>[2x]SMEMRAVVLAGFGGLNKLRLFRKAMPEPQDGELKIRVKACGLNFIDLMVRQGNIDNPPKTPLVPGFECSGIVEALG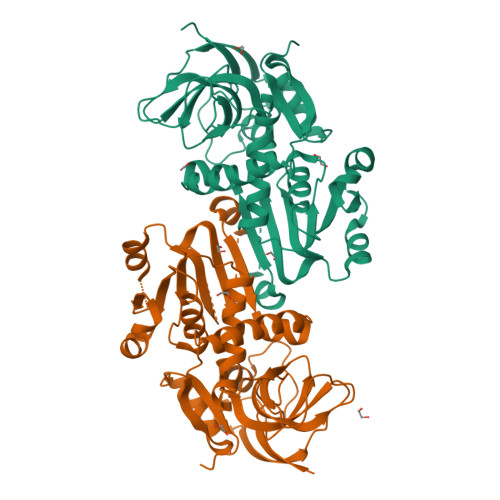DSVKGYEIGDRVMAFVNYNAWAEVVCTPVEFVYKIPDDMSFSEAAAFPMNFVTAYVMLFEVANLREGMSVLVHSAGGGVGQAVAQLCSTVPNVTVFGTASTFKHEAIKDSVTHLFDRNADYVQEVKRISAEGVDIVLDCLCGDNTGKGLSLLKPLGTYILYGSSNMVTGETKSFFSFAKSWWQVEKVNPIKLYEENKVIAGFSLLNLLFKQGRAGLIRGVVEKLIGLYNQKKIKPVVDSLWALEEVKEAMQRIHDRGNIGKLILDVEKTPTPL> MSFRTHLESVVNQVEGALACSVMGFDGISVDTFQKDESAELDLNGAWVEYANLLTQLRNAAETLKTGTVSEVSVNSEKVLTVMRLVSPDYFLVLALHADGNFGKGRYVLRVTAPKVRAEL

Mutual gliding motility protein C (MglC), a paralog of GTPase-activating protein Mutual gliding motility protein B (MglB), is a member of the polarity module involved in regulating motility. MglC is required for polarity reversal and interacts with MglB and RomR. The crystal structure revealed that, despite sharing <9% sequence identity, both MglB and MglC adopt a Regulatory Light Chain 7 family fold. Using isothermal titration calorimetry and size-exclusion chromatography, we show that MglC binds MglB in 2:4 stoichiometry with submicromolar range dissociation constant.

There was no good structural template to use as a model for solving structure using molecular replacement. The closest homologue available at RCSB PDB shared ∼8% sequence identity. So, we solved the crystal structure using Selenomethionine Single-wavelength anomalous diffraction (Se-SAD) experimental phasing technique at 1.85 Å resolution. MglC crystallized in P6522 space group (a = 96.69 Å, b = 96.69 Å, c = 58.28 Å, α = 90°, β = 90°, γ = 120°) with one molecule in an asymmetric unit. The final refined model contains all 120 residues of MglC. The crystal structure revealed the typical RLC7 fold (α1β1β2α2β3α3). MglC monomer contains five antiparallel β-strands sandwiched between three α-helices. We also observed an electron density for a metal ion in the crystal structure having a square pyramidal geometry. We placed Na+ which is coordinated by two water molecules and main chain oxygen atoms of L64, T66, and V69. The native and Se-SAD structures superpose well with r.m.s.d. of 0.144.5'-O-[(R)-hydroxy{[(S)-hydroxy(phosphonoamino)phosphoryl]oxy}phosphoryl]uridine 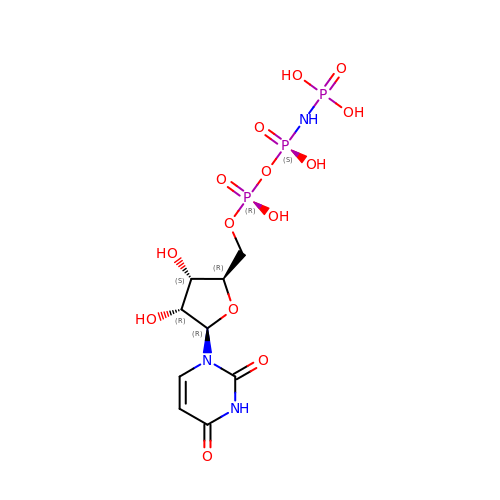| C9 H16 N3 O14 P3 | MCBVWUSULWKVON-XVFCMESISA-N> STQAATASSRNSCAADDKATEPLPKDCPVSSYNEWDPLEEVIVGRAENACVPPFTIEVKANTYEKYWPFYQKQGGHYFPKDHLKKAVAEIEEMCNILKTEGVTVRRPDPIDWSLKYKTPDFESTGLYSAMPRDILIVVGNEIIEAPMAWRSRFFEYRAYRSIIKDYFHRGAKWTTAPKPTMADELYNQDYPIHSVEDRHKLAAQGKFVTTEFEPCFDAADFIRAGRDIFAQRSQVTNYLGIEWMRRHLAPDYRVHIISFKDPNPMHIDATFNIIGPGIVLSNPDRPCHQIDLFKKAGWTIITPPTPIIPDDHPLWMSSKWLSMNVLML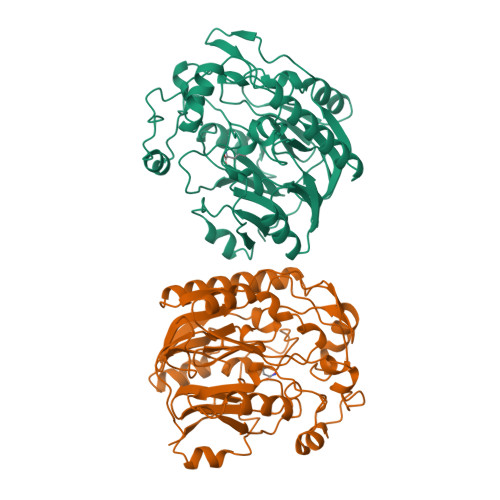DEKRVMVDANEVPIQKMFEKLGITTIKVNIRNANSLGGGFHCWTCDVRRRGTLQSYLD> MALAKRIIAALIVKDGRVVKGSNFENLRDSGDPVELGKFYSEIGIDELSFADITASVEKRKTMLELVEKVAEQIDIPFTVGGGIHDFETASELILRGADKVEINTAAVENPSLITQIAQTFGSQAVVVYIAAKRVDGEFMVFTYSGKKNTGILLRDWVVEVEK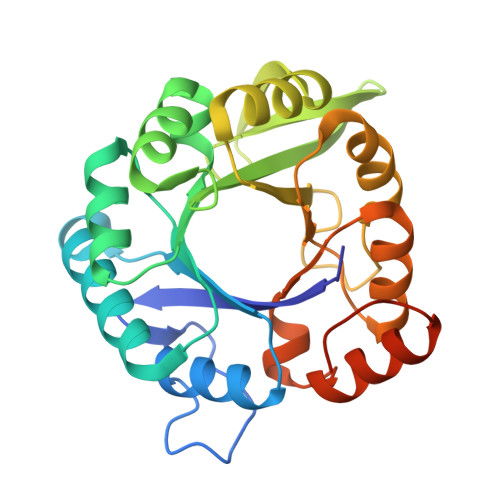RGAGEIVLGSIDRLGTKSGYDTEMIRFVRPLTTLPIIAHGGAGKMEHFLEAFLAGADAAKANSVLHFREIDVRELKEYLKKHGVNVRLEGLGSLEHHHHHH> MDGYKVEVGKNAYLPCSYTLPTSGTLVPMCWGKGFCPWSQCTNELLRTDERNVTYQKSS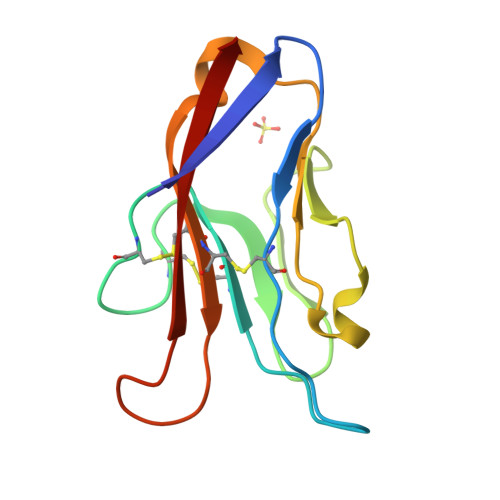RYQLKGDLNKGDVSLIIKNVTLDDHGTYCCRIQFPGLMNDKKLELKLDIK>[4x]MAKIKNPILTGFHPDPSICRVGDDYYIAVSTFEWFPGVRIYHSKDLKNWRLVARPLNRLSQLNMIGNPDSG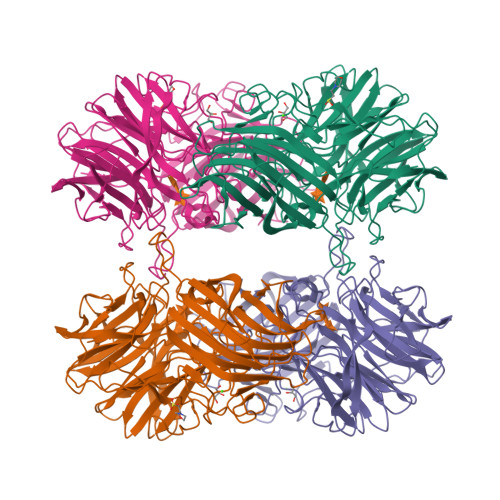GVWAPHLSYSDGKFWLIYTDVKVVEGQWKDGHNYLVTCDTIDGAWSDPIYLNSSGFDPSLFHDEDGRKYLVNMYWDHRVDHHPFYGIVLQEYSVEQKKLVGEPKIIFKGTDLRITGGPHLYKINGYYYLLTAEGGTRYNHAATIARSTSLYGPYEVHPDNPLLTSWPYPRNPLQKAGHASIVHTHTDEWFLVHLTGRPLPREGQPLLEHRGYCPLGRETAIQRLEWKDGWPYVVGGNGPSLEIDGPSVEEVSWEKDYDEKDDFDGDTLNHHFQTLRIPLGEDIATLKARPGHLRLYGRESLTSRFTQAFVARRWQHFHFVAETKVSFRPTTFQQSAGLVNYYNTQNWTTLQITWHEEKGRILELMTCDHLVVDQPLRGREIVVPDDIEYVYLRVTVQATTYKYSYSFDGMNWIDLPVTFESYKLSDDYIKSRAAFTGAFVGMHCRDGSGQNNYADFDYFLYKEL(2S)-sulfonatepropionyl-CoA | 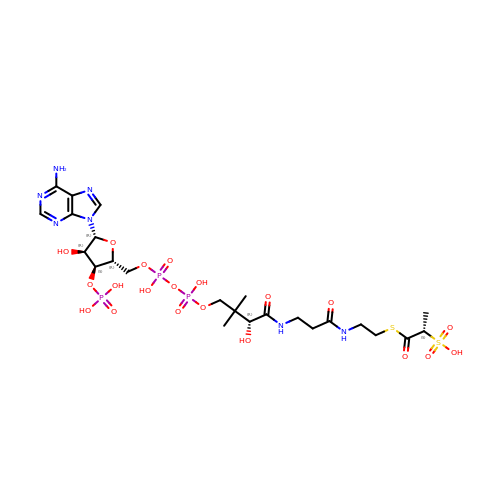C24 H40 N7 O20 P3 S2 | GJGCZNMXHKQRSE-IBNUZSNCSA-N6-{[(3R,4S)-4-(2-{[2-(3-fluorophenyl)ethyl]amino}ethoxy)pyrrolidin-3-yl]methyl}-4-methylpyridin-2-amine 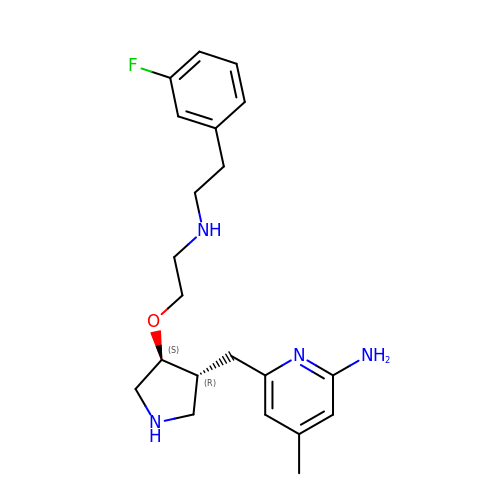| C21 H29 F N4 O | NESZTSPBRDBHCW-YLJYHZDGSA-N>GPNLELLESFGQNYPEEADGTLDCISMALTCTFNRWGTLLAVGCNDGRIVIWDFLTRGIAKIISAHIHPVCSLCWSRDGHKLVSASTDNIVSQWDVLSGDCDQRFRFPSPILKVQYHPRDQNKVLVCPMKSAPVMLTLSDSKHVVLPVDDDSDLNVVASFDRRGEYIYTGNAKGKILVLKTDSQDLVASFRVTTGTSN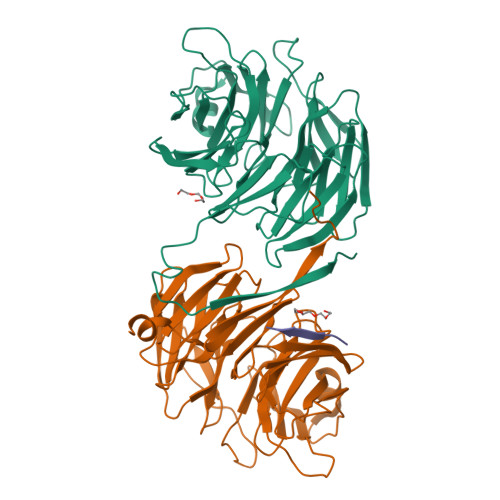TTAIKSIEFARKGSCFLINTADRIIRVYDGREILTCGRDGEPEPMQKLQDLVNRTPWKKCCFSGDGEYIVAGSARQHALYIWEKSIGNLVKILHGTRGELLLDVAWHPVRPIIASISSGVVSIWAQNQVENWSAFAPDFKELDENVEYEERESEFDIEDEDKSEPKQTGADAAEDEEVDVTSV[2x];> EPKQTG> MASWSHPQFEKGAENLYFQSNATEKLRLDIPVLLPGLPDSSDPCVERLLSELRGKEGVEAAHIKTANVDSDSQICVHYDPAAISLARIRELVTSTGAVISSR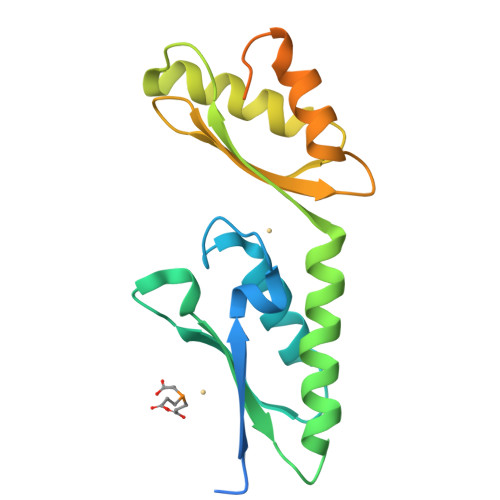FGHVLWQLKGVWHERRARTVASQLRALPGVIEAEVSASGIARVEFDNDRISAAGIEQALSKRGLAPVEIGARKSGHADHEHREGVKDHAHGEGEGHEAHAHGSVFG>MEESSEIKVETNISKTSWIRSSMAASGKRVSKALSYITGEMKECGEGLKDKSPVFQFFDWVLRGTSQVMFVNNPLSGILIILGLFIQNPWWAISGCLGTIMSTLTALILSQDKSAIAAGFHGYNGVLVGLLMAVFSDKGDYYWWLLLPVIIMSMSCPILSSALGTIFSKWDLPVFTLPFNITVTLYLAATGHYNLFFPTTLLQPASAMPNITWSEVQVPLLLRAIPVGIGQVYGCDNPWTGGIFLIALFISSPLICLHAAIGSTMGMLAALTIATPFDSIYFGLCGFNSTLACIAIGGMFYVITWQTHLLAIACALFAAYLGAALANMLSVFGLPPCTWPFCLSALTFLLLTTNNPAIYKLPLSKV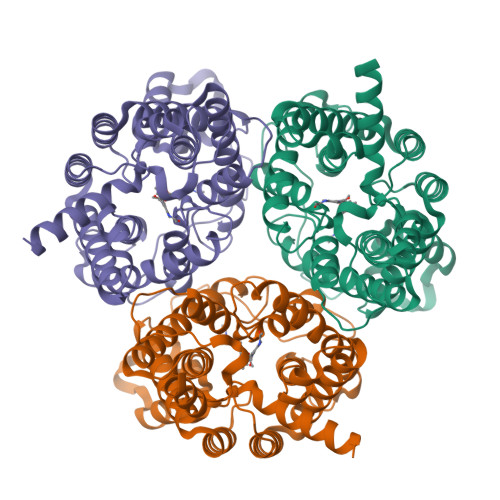TYPEANRIYYLSQERNRRASIITKYQAYDVS[3x]> MKNDRTLQAIGRQLKAMGCERFDIGVRDATTGQMMNREWSAAEVLQNTPWLKRMNAQGNDVYIRPAEQERHGLVLVDDLSEFDLDDMKAEGREPALVVETSPKNYQAWVKVADAAGGELRGQIARTLASEYDADPASADSRHYGRLAGFTNRKDKHTTRAGYQPWVLLRESKGKTATAGPALVQQAGQQIEQAQRQ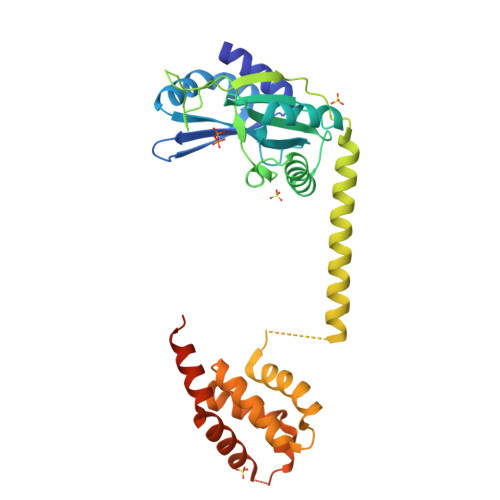QEKARRLASLELPERQLSRHRRTALDEYRSEMAGLVKRFGDDLSKCDFIAAQKLASRGRSAEEIGKAMAEASPALAERKPGHEADYIERTVSKVMGLPSVQLARAELARAPAPRQRGMDRGGPDFSM>[2x]QSACTLQPETHPPLTWQKCSSGGTCTQQTGSVVIDANWRWIHATNSSTSCYDGNTWSSTLCPDNETCTKNCCLDGAAYASTYGVTTSGDSLTIGFVTQSAQKNVGARLYLMANDTTYQEFTLLGNEFSFDVDVSQLPCGLNGALYFVSMDADGGVSKYPTNTAGAKYGTGYCDSQCPRDLKFING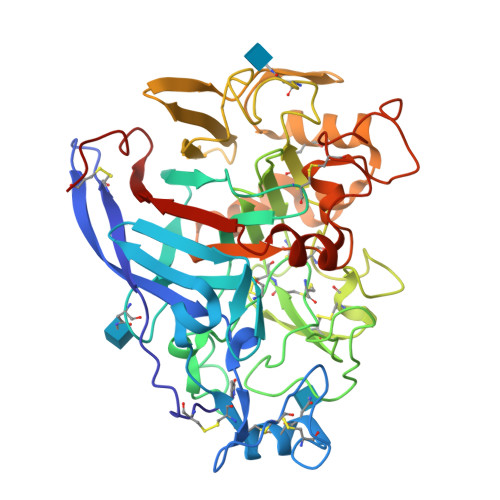QANVEGWEPSTNNANTGIGGHGSCCSEMDIWEANSISEALTLHPCTTVGQEICEGDGCGGTYSKNRYGGPCDPDGCDWNPYRLGNTSFYGPGPSFTLDTTKKLTVVTQFKPSGAINRYYVQNGVTFQQPNAELGSYSGNELNDDYCYAEEAEFGGSSFSDKGGLTQFKKATSGGMVLVMSLWDDYYANMLWLDSTYPTNETSSTPGAVRGSCSTSSGDPAQVESQFPNAKVTFSNIKFGPIGSTGNPSG> MEHTIAVIPGSFDPITYGHLDIIERSTDRFDEIHVCVLKNSKKEGTFSLEERMDLIEQSVKHLPNVKVHQFSGLLVDYCEQVGAKTIIRGLRAVSDFEYELRLTSMNKKLNNEIETLYMMSSTNYSFISSSIVKEVAAYRADISEFVPPYVEKALKKKF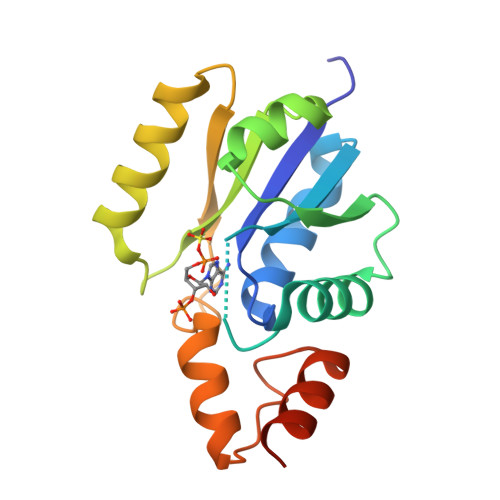KLEHHHHHH> SSLENVVYNLVNAGHFDGRAGE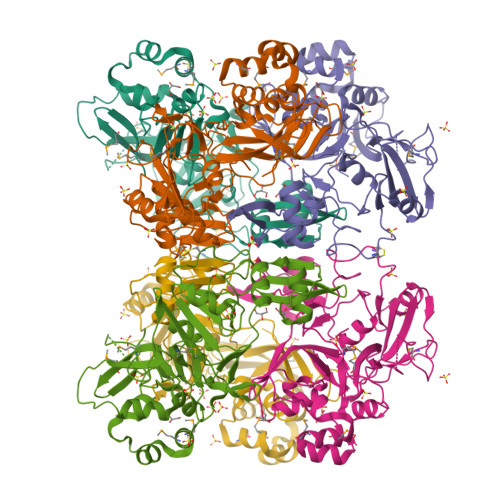LPCAVIGEKVIAKIQNEDVVVFKNNTPFPTNVAVELFAKRSIRPHPELKLFRNLNIDVCWSHVLWDYAKDSVFCSSTYKVCKYTDLQCIESLNVLFDGRDNGALEAFKKCRNGVYINTTKIKSLSMIKGPQRADLNGVVVEKVGDSDVEFWFAVRKDGDDVIFSRTGSLEPSHYRSPQGNPGGNRVGDLSGNEALARGTIFTQSRLLSSFTPRSEMEKDFMDLDDDVFIAKYSLQDYAFEHVVYGSFNQKIIGGLHLLIGLARRQQKSNLVIQEFVTYDSSIHSYLITDENSGSSKSVCTVIDLLLDDFVDIVKSLNLKCVSKVVNVNVDFKDFQFMLWCNEEKVMTF>GCUACGAAGGAAGGAUUGGUAUGUGGUAUAUUCGUA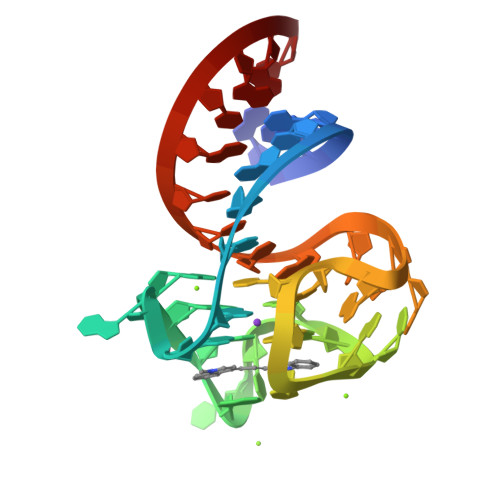GC[2x]We have identified a novel gene that is associated with changes in virulence, CNAG_02591 (hypervirulence-associated protein 1, HVA1), through gene expression microarray analysis that compared two mouse-passaged strains to the pre-passage H99W strain. The HVA1 gene is predicted to contain 3 exons separated by two introns that encode a 75 amino acid protein. No known protein domains or homologous gene families exist for this gene. Metabolomics analysis suggests that when HVA1 is absent there is a block in the citric acid cycle, while structural analysis of the Hva1 protein suggests a potential interaction with NADPH.

To gain insight into the potential function of HVA1, the structure of the Hva1 protein was solved by X-ray crystallography and refined to highly acceptable accuracy. The three dimensional architecture of each Hva1 monomer was predominantly β-stranded. There were seven β-strands of varying lengths with five forming interdigitating antiparallel hydrogen bonds to create a semi-cylindrical barrel-like twisted β-sheet. In addition, this small protein also contained one unconnected α-helix. Overall, the monomeric structure of Hva1 resembled a 6-fingered human palm with the α-helix forming the thumb. The crystal structure further revealed that the protein crystallized in a P1 space group with two Hva1 monomers that are related by a non-crystallographic two-fold symmetry. The interface is very extensive as the “thumb” helix of the first monomer is inserted firmly into the “fingers” forming the semi-cylindrical barrel of the second monomer. The monomers are connected by extensive polar and apolar interactions. Although the observed 2-fold association between the two Hva1 monomers may be a crystallographic artifact, the potential for these interacting surfaces to attract ligands and binding partners cannot be completely ruled out. The region corresponding to the monomer-monomer interface of Hva1 was occupied by a bound nicotinamide adenine dinucleotide phosphate (NADP) ligand in DHFR-NADP complex.

>[2x]GSMSVQDKQGQNINVGDTVYTPYRGGKHEGQVADIVTTKEEAAEKGVKNPPKVLFTDQNNKDVAHNPGTLTDLDKQK> APKDNTWYTGAKLGWSQYHDTGFINNNGPTHENKLGAGAFGGYQVNPYVGFEMGYDWLGRMPYKGSVENGAYKAQGVQLTAKLGYPITDDLDIYTRLGGMVWRADTYSNVYGKNHDTGVSPVFAGGVEYAITPEI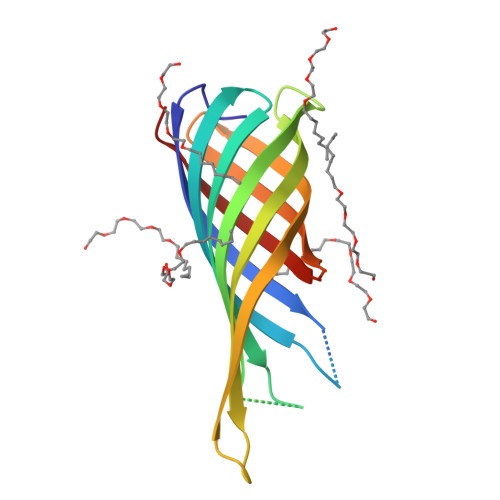ATRLEYQWTNNIGDAHTIGTRPDNGMLSLGVSYRFG> SNASKMSDVKCTSVVLLSVLQQLRVESSSKLWAQCVQLHNDILLAKDTTEAFEKMVSLLSVLLSMQGAVDINKLCEEMLDNRATLQ;> EDKRAKVTSAMQTMLFTMLRKLDNDALNNIINNARDGCVPLNIIPLTTAAKLMVVIPDYNTYKNTCDGTTFTYASALWEIQQVVDADSKIVQLSEISMDNSPNLAWPLIVTALRANSAVKLQ

SARS-CoV-2 RdRp, also referred to as nonstructural protein 12 (Nsp12), is the catalytic center of the macromolecular complex frequently referred to as the replication transcription complex (RTC). The RTC is essential for virus replication because it makes copies of genomic and subgenomic RNAs and polymerizes antisense RNA. In SARS-CoV-2, besides RdRp (Nsp12), the RTC involves nonstructural proteins Nsp7, Nsp8, and others. Nsp12 is the largest component of the complex, and Nsp7 and Nsp8 are considered cofactors.

To provide insights into the structures, key residues of association, and multimeric state between the SARS-CoV-2 RTC’s cofactors, we solved high-resolution crystal structures of Nsp7 bound to Nsp8. Crystals of Nsp7/8A were shown to have a truncated N-terminus (at residue Glu78) for Nsp8. In all of our crystal forms, the heterodimer formed between Nsp7 and 8 places Nsp7 near the half β-barrel-like domain of Nsp8 with the N-terminal helix of Nsp8 extended and pointing away (approximate dimensions of 40 × 40 × 46 Å). The similarity between all heterodimers in all our crystal forms is remarkable, with a root mean square deviation of 0.82 Å for 184 aligned Cα atoms despite different unit cell dimensions, different space groups, and different asymmetric units. In contrast to previously reported Nsp7/8 structures from other coronaviruses, in all three of our structures, either as in the asymmetric content or symmetry related, a heterotetramer or a dimer of heterodimers is present as an elongated, thick rod shape of 40 × 92 Å. The differing crystal forms show only slight variation in the packing of Nsp7/8 heterodimers to form heterotetramers. In Nsp7/8A, the tetramers are formed by the crystallographic twofold rotational symmetry. The heterotetramer interface involves a total of six helices: α1 and α2 of Nsp7 and their symmetry mates (twofold rotation) α1′ and α2′ and α1 of Nsp8 and the symmetry mate α1′. The tetramer interface is not as extensive as that of the dimer having 1813 Å2 with 73% being hydrophobic.3-fluoranyl-~{N}-[(~{E})-(5-pyridin-2-ylsulfanylfuran-2-yl)methylideneamino]benzamide 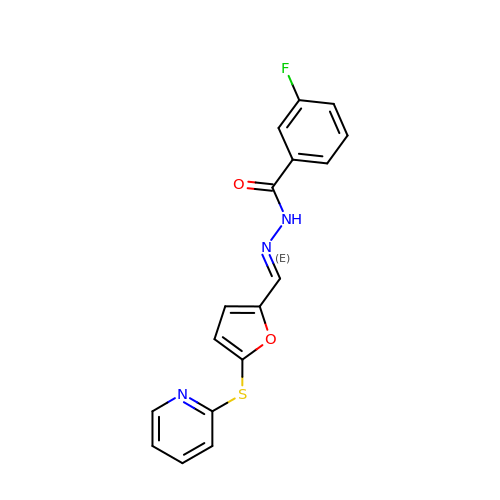| C17 H12 F N3 O2 S | VDKNIVFIPSLUFD-RGVLZGJSSA-N> QTVEAMAQGLPAPSYWKNERGSELLIWSANSGTI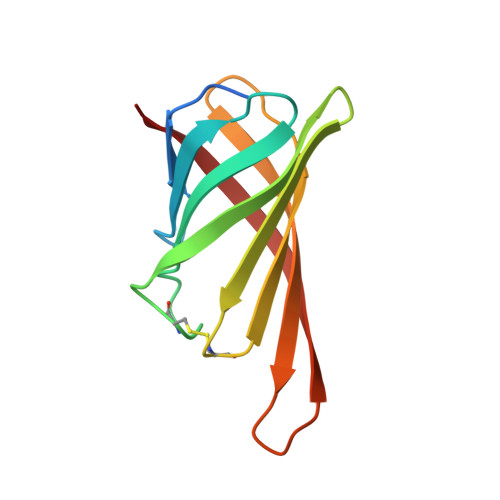QGTFTNHAQGFACQGIPYPAAGSVSPTGLYFVVTFAQCNSFTRWVGTIKGSQMPTSWTLFYVDNKGKPSRLKGGDIFTRVW> KDMFNTKSSNGKLRIEDASHNARKLGLAPSSTDEKKIRDLYG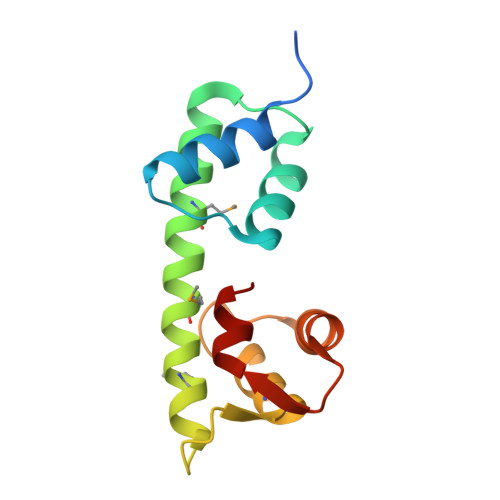DSLTYEQYLEYLTMCVHDRDNMEELIKMFSHFDNNSSGFLTKNQMKNILTTWGDALTEQEANDALNAFSSEDRINYKLFCEDIL6-carboxy methyl-4-hydroxy-2-pyridinol | C8 H9 N O4 | 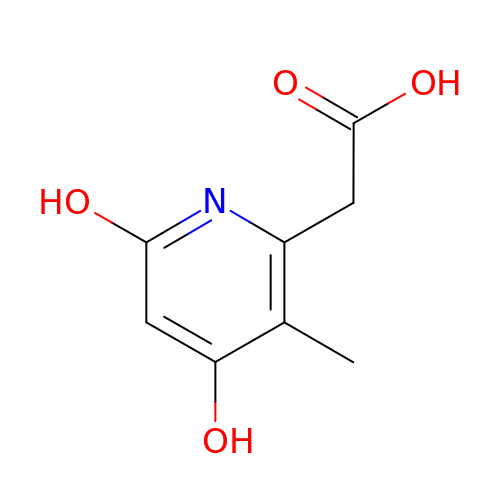MGGXBHMHJPCYSF-UHFFFAOYSA-N> MLVSKFENSVKNSNKNYFTINGLMGYYFENDFFNLNIISPTLDGNLTFSKEDINSILGNKIIKSARWIGLIKPSITGEYILSTNSPNCRVELNGEIFNLSLNTSNTVNLIQGNVYDIRIEQLMSENQLLKNYEGIKLYWETSDIIKEIIPSEVLLKPNYSNTNEKSKFIPNNTLFSNAKLKANANRDTDRDGIPDEWEINGYTVMNQKAVAWDDKFAANGYKKYVSNPFKPCTANDPYTDFEKVSGQIDPSVSMVARDPMISAYPIVGVQMERLVVSKSETITGDSTKSMSKSTSHSSTNINTVGAEVSGSLQLAGGIFPVFSMSASANYSHTWQNTSTVDDTTGESFSQGLSINTAESAYINPNIRYYNTGTAPVYNVTPTTTIVIDKQSVATIKGQESLIGDYLNPGGTYPIIGEPPMALNTMDQFSSRLIPINYNQLKSIDNGGTVMLSTSQFTGNFAKYNSNGNLVTDGNNWGPYLGTIKSTTASLTLSLPDQTTQVAVVAPNFSDPEDKTPRLTLEQALVKAFRLEKKNGKFYFHGMEISANQKIQVFLDRNTNVDFENQLKNTANKDIMNCIIKRNMNILVKVITFKENISSINIINDTNFGVESMTGLSKRIKGNDGIYRASTKSFS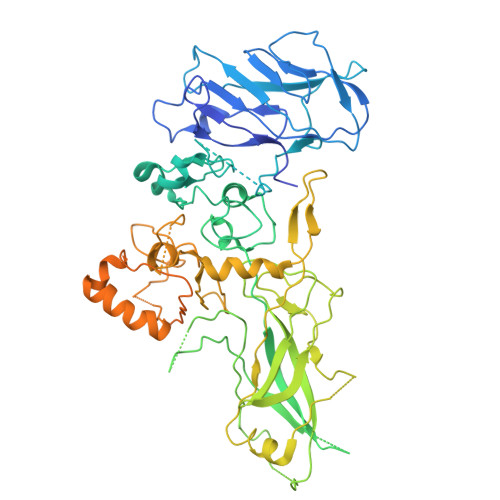FKSKEIKYPEGFYRMRFVIQSYEPFTCNFKLFNNLIYSNSFDIGYYDEFFYFYCNGSKSFFDISCDIINSINRLSGVFLIELDKLII>[2x]MGHHHHHHHHMATLTAKNLAKAYKGRRVVEDVSLTVNSGEIVGLLGPNGAGKTTTFYMVVGIVPRDAGNIIIDDDDISLLPLHARARRGIGYLPQEASIFRRLSVYDNLMAVLQIRDDLSAEQREDRANELMEEFHIEHLRDSMGQSLSGGERRRVEIARALAANPKFI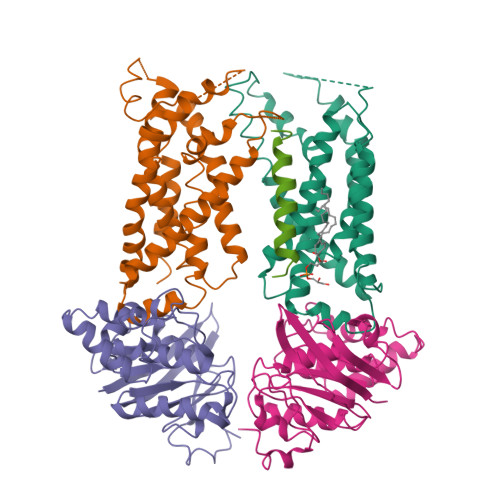LLDEPFAGVDPISVIDIKRIIEHLRDSGLGVLITDHNVRETLAVCERAYIVSQGHLIAHGTPTEILQDEHVKRVYLGEDFRL;> MWSHPQFEKENLYFQGGMSKARRWVIIVLSLAVLVMIGINMAEKDDTAQVVVNNNDPTYKSEHTDTLVYNPEGALSYRLIAQHVEYYSDQAVSWFTQPVLTTFDKDKIPTWSVKADKAKLTNDRMLYLYGHVEVNALVPDSQLRRITTDNAQINLVTQDVTSEDLVTLYGTTFNSSGLKMRGNLRSKNAELIEKVRTSYEIQNKQTQP;> MIIIRYLVRETLKSQLAILFILLLIFFCQKLVRILGAAVDGDIPANLVLSLLGLGVPEMAQLILPLSLFLGLLMTLGKLYTESEITVMHACGLSKAVLVKAAMILAVFTAIVAAVNVMWAGPWSSRHQDEVLAEAKANPGMAALAQGQFQQATNGSSVLFIESVDGSDFKDVFLAQIRPKGNARPSVVVADSGHLTQLRDGSQVVTLNQGTRFEGTALLRDFRITDFQDYQAIIGHQAVALDPNDTDQMDMRTLWNTDTDRARAELNWRITLVFTVFMMALMVVPLSVVNPRQGRVLSMLPAMLLYLLFFLIQTSLKSNGGKGKLDPTLWMWTVNLIYLALAIVLNLWDTVPVRRLRASFSRKGAV;> MQPFGVLDRYIGKTIFTTIMMTLFMLVSLSGIIKFVDQLKKAGQGSYDALGAGMYTLLSVPKDVQIFFPMAALLGALLGLGMLAQRSELVVMQASGFTRMQVALSVMKTAIPLVLLTMAIGEWVAPQGEQMARNYRAQAMYGGSLLSTQQGLWAKDGNNFVYIERVKGDEELGGISIYAFNENRRLQSVRYAATAKFDPEHKVWRLSQVDESDLTNPKQITGSQTVSGTWKTNLTPDKLGVVALDPDALSISGLHNYVKYLKSSGQDAGRYQLNMWSKIFQPLSVAVMMLMALSFIFGPLRSVPMGVRVVTGISFGFVFYVLDQIFGPLTLVYGIPPIIGALLPSASFFLISLWLLMRKS>MGSSHHHHHHENLYFQGGMTLFTENDLLNNSYKSIQKSYHFSENQAAKNILEQAYKNYDKNKIYDIFLSHSFLDARKILGLKNYIEGLGYSVYVDWIEDKQLDRSKVSKETAGILRERMQSCKSLFFAISENSDHSLWMPWELGYFDGIKQKVAILPVLKSSYDDSYNGQEYLGLYPYVAKGTIINSTQEEIWIHSSQKQYVRFRNWLQ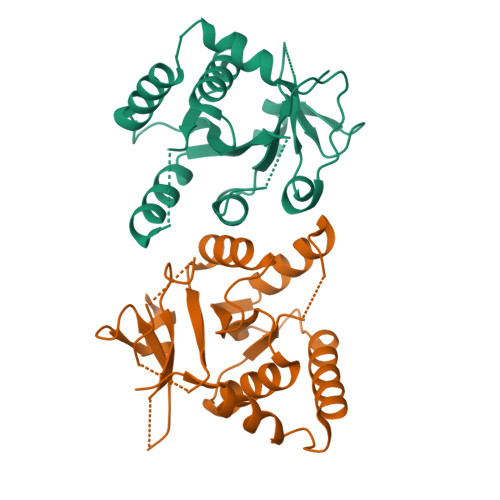QN[2x]>MPENYTPAAAATGTWTEEEIRHQPRAWIRSLTNIDALRSALNNFLEPLLRKENLRIILTGAGTSAFIGDIIAPWLASHTGKNFSAVPTTDLVTNPMDYLNPAHPLLLISFGRSGNSPESVAAVELANQFVPECYHLPITCNE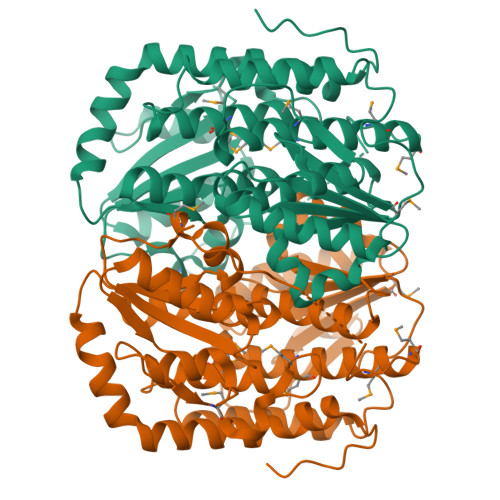AGALYQNAINSDNAFALLMPAETHDRGFAMTSSITTMMASCLAVFAPETINSQTFRDVADRCQAILTSLGDFSEGVFGYAPWKRIVYLGSGGLQGAARESALKVLELTAGKLAAFYDSPTGFRHGPKSLVDDETLVVVFVSSHPYTRQYDLDLLAELRRDNQAMRVIAIAAESSDIVAAGPHIILPPSRHFIDVEQAFCFLMYAQTFALMQSLHMGNTPDTPSASGTVNRVVQGVIIHPWQA[6x]> CGC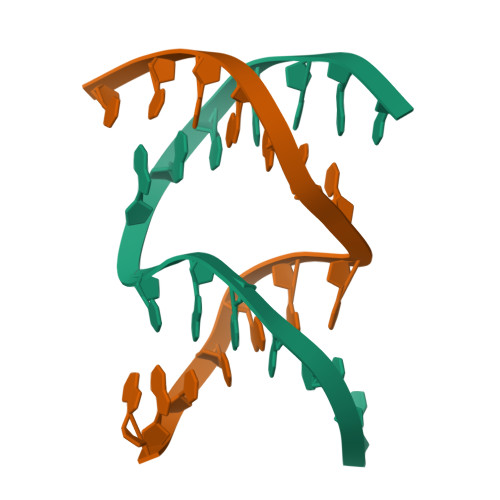TGGTGGTTCGA;> GACCAGCCGAACCT> AVLTQTQIDSILADLAHHTDTTEHITEMGVSIYKTLFAAHPEYISYFSKLQGLTKDNVGQSEGIRYYGRTLGEELIRLLKAASNPSVLEERIVQGAKDHKARPVTKDQFT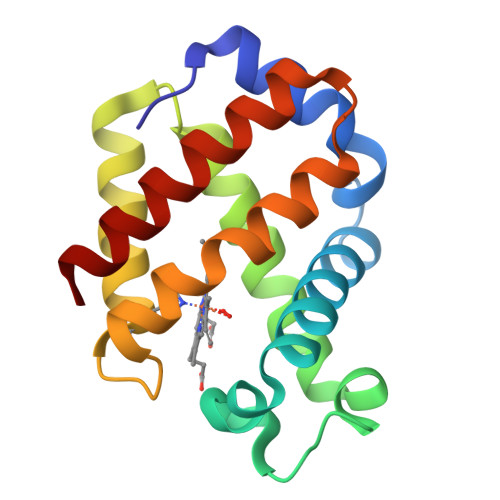GAAPIFIKFFQGLLKKQEDKDAIEKFLLHVMQAIAAKM>[3x]ACVF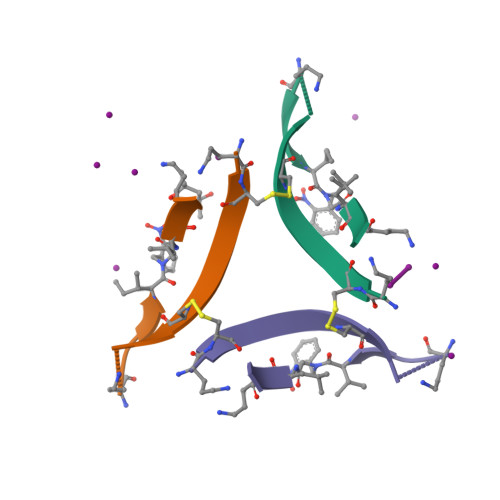FCEDAAIIXLAV phenanthridin-6(5H)-one | C13 H9 N O | 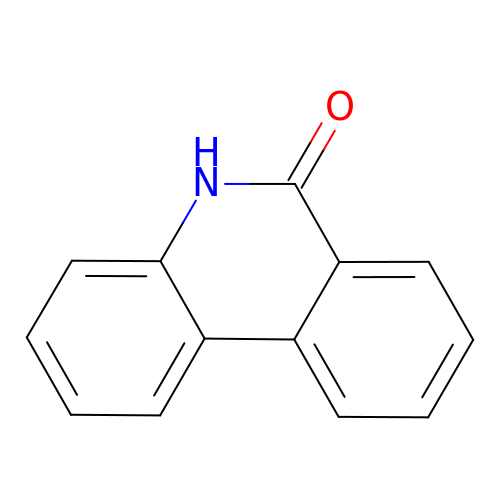RZFVLEJOHSLEFR-UHFFFAOYSA-N>[2x]MGSDKIHHHHHHMDLWKLYQPGTPAAIVAWGQLGTAHAKTTYGLLRHSRLFKPVCVVAEHEGKMASDFVKPVRYDVPVVSSVEKAKEMGAEVLIIGVSNPG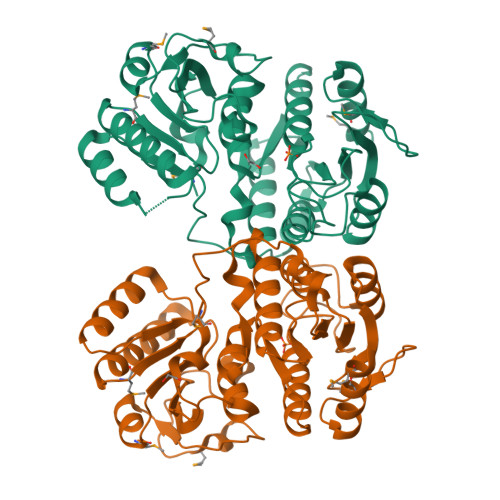GYLEEQIATLVKKALSLGMDVISGLHFKISQQTEFLKIAHENGTRIIDIRIPPLELDVLRGGIYRKKIKVVGVFGTDCVVGKRTTAVQLWERALEKGIKAGFLATGQTGILIGADAGYVIDAVPADFVSGVVEKAVLKLEKTGKEIVFVEGQGALRHPAYGQVTLGLLYGSNPDVVFLVHDPSRDHFESFPEIPKKPDFEEERRLIETLSNAKVIGGVSLNGGFETDLPVYDPFNTDDLDEMLERAMVW(S)-2-(2-((2H-tetrazol-5-yl)methoxy)-4-methylphenyl)-1-(4-chlorophenyl)-6,7-diethoxy-1,2-dihydroisoquinolin-3(4H)-one | C28 H28 Cl N5 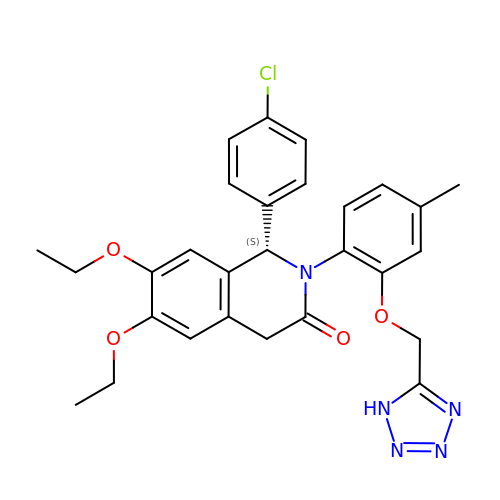O4 | FOCZOWVAISYOAB-NDEPHWFRSA-N>[2x]MSDKDSKNTPQVPEKLGLSRRGFLGASAVTGAAVAATALGGAVMTRESWAQAVKESKQKIHVGPGELDDYYGFWSGGHQGEVRVLGVPSMRELMRIPVFNVDSATGWGLTNESRHIMGDSAKFLNGDCHHPHISMTDGKYDGKYLFINDKANSRVARIRLDIMKCDKMITVPNVQAIHGLRL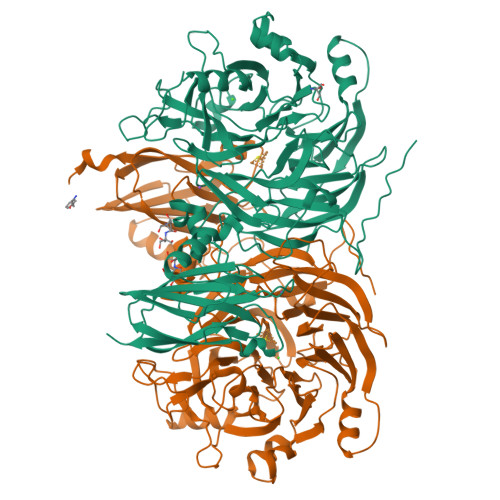QKVPHTKYVFANAEFIIPHPNDGKVFDLQDENSYTMYNAIDAETMEMAFQVIVDGNLDNTDADYTGRFAAATCYNSEKAFDLGGMMRNERDWVVVFDIHAVEAAVKAGDFITLGDSKTPVLDGRKKDGKDSKFTRYVPVPKNPHGCNTSSDGKYFIAAGKLSPTCSMIAIDKLPDLFAGKLADPRDVIVGEPELGLGPLHTTFDGRGNAYTTLFIDSQVVKWNMEEAVRAYKGEKVNYIKQKLDVHYQPGHLHASLCETNEADGKWLVALSKFSKDRFLPVGPLHPENDQLIDISGDEMKLVHDGPTFAEPHDCIMARRDQIKTKKIWDRNDPFFAPTVEMAKKDGINLDTDNKVIRDGNKVRVYMTAMAPAFGVQEFTVKQGDEVTVTITNIAQIEDVSHGFVVVNHGVSMEISPQQTSSITFVADKPGLHWYYCSWFCHALHMEMVGRMMVEPAWSHPQFE> SNVEPVGRLHIFSGAHGPEKDFPLHLGKNVVGRMPDCSVALPFPSISKQHAEIEILAWDKAP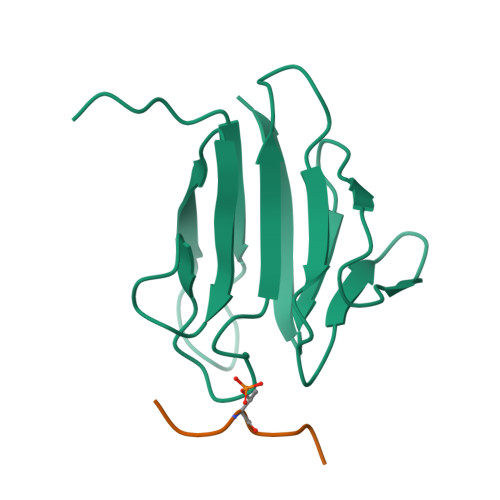ILRDCGSLNGTQILRPPKVLSPGVSHRLRDQELILFADLLCQYHRLDVSLP;> MEDTQAID> MDIEIAPQRQEPLPYVPEGYSPFQQDDIEKLKTFNSPYK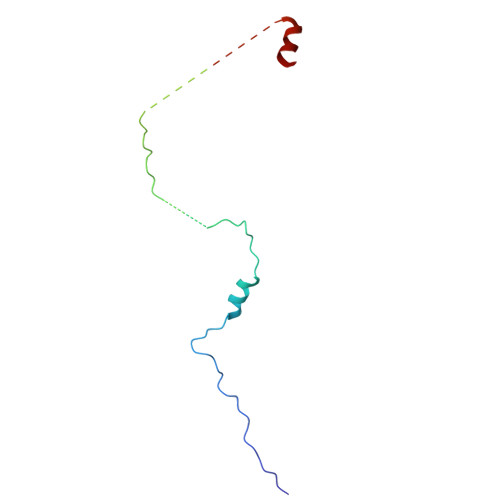LDLEDEDDTPDKVDLLPLEQIDEEGEKDETECITRNQEEGAALPLLSKNFKEVAAVPTMELVYSEEGLDPEELEDLVT5-[(2-anilino-2-oxoethyl)(methyl)amino]-N-hydroxypentanamide | C14 H21 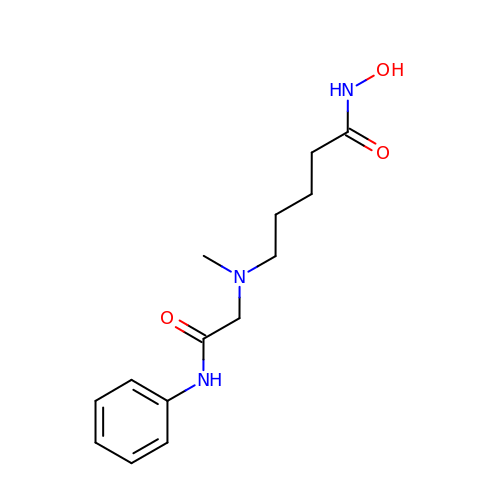N3 O3 | ZPXKDKFZPZUKPI-UHFFFAOYSA-N Here we report that pyrrolysyl-tRNA synthetase (PylRS) and certain PylRS variants accept α-hydroxy, α-thio and N-formyl-l-α-amino acids, as well as α-carboxy acid monomers that are precursors to polyketide natural products. Here we report that the tolerance of MmPylRS for substrates with multiple alternative substituents in place of the α-amine extends to Methanomethylophilus alvus PylRS (MaPylRS)38,39 as well as MaPylRS variants (N166A V168L, MaFRS1 and N166A V168K, MaFRS2) that recognize diverse l-phenylalanine derivatives. We expressed and purified an MaPylRS variant containing these mutations (MaFRSA with N166A and V168A) and demonstrated using RNAse A and intact tRNA analysis that it shows high activity for derivatives of malonic acid 14 carrying m-CH3 (17), m-CF3 (18) and m-Br substituents and low activity for l-Phe. In vivo studies using traditional and engineered E. coli strains confirmed that MaFRSA supports the biosynthesis of model proteins containing internal, aromatic, α-hydroxy acid monomers. This work describes the first aaRSs that accept α-thio acids and α-carboxy acids that could support carbon–carbon bond formation within the ribosome.

To better understand how 2-BMA substrates are accommodated by the MaFRSA active site, we solved the crystal structure of MaFRSA bound to both m-CF3-2-BMA and the non-hydrolysable ATP analogue adenosine 5′-(β,γ-imido)triphosphate (AMP-PNP). The structure was refined at 1.8 Å resolution with clear substrate density for m-CF3-2-BMA visible in the electron density map. MaFRSA crystallized with two protein chains in the asymmetric unit and an overall architecture resembling previously published PylRS structures. The two protein chains in the asymmetric unit are not identical and interact with different orientations of m-CF3-2-BMA. In chain A, the pro-S carboxylate accepts a hydrogen bond from the backbone amides of Leu121 and Ala122 and the phenolic -OH of Tyr206. A hydrogen bond from the Arg150 guanidinium positions the pro-R carboxylate for nucleophilic attack with a distance of 2.7 Å between the carboxy oxygen and the α-phosphorus of AMP-PNP. In chain B, the orientation of m-CF3-2-BMA is flipped relative to the conformation bound to chain A. The pro-R carboxylate accepts a hydrogen bond from the backbone amides of Leu121 and Ala122 and the phenolic -OH of Tyr206, as seen for the pro-S carboxylate in chain A. However, in chain B, the pro-S carboxylate is rotated away from AMP-PNP and towards Tyr206, resulting in loss of the hydrogen bond to Arg150 and a longer distance of 3.9 Å between the carboxy oxygen and the α-phosphorus of AMP-PNP. The two alternative poses of m-CF3-2-BMA in chains A and B correspond to a rotation of ~120° about the Cα–Cβ bond of the substrate that largely maintains interactions with the m-CF3-2-BMA side chain but alters the placement of the reacting carboxylate.

>[2x]GSHMTVKYTDAQIQRLREYGNGTYEQKVFEDLASRDAAFSKEMSVASTDNEKKIKGMIANPSRHGLTQLMNDIADALVAEGFIEVRTPIFISKDALARMTITEDKPLFKQVFWIDEKRALRPMLAPNLYSVMRDLRDHTDGPVKIFEMGSCFRKESHSGMHLEEFTMLALADMGPRGDATEVLKNYISVVMKAAGLPDYDLVQEESDVYKETIDVEINGQEVCSAAVGPHYLDAAHDVHEPWSGAGFGLERLLTIREKYSTVKKGGASISYLNGAKIN6-azanyl-4-(3-methylphenyl)-1~{H}-pyrrolo[2,3-b]pyridine-3-carbonitrile | C15 H12 N4 | 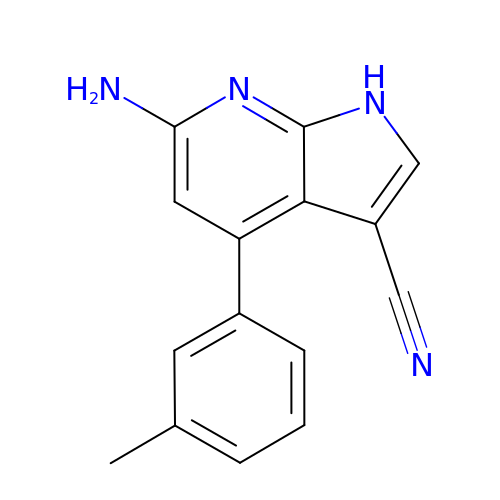KWTGXMXCSXFSJX-UHFFFAOYSA-N> CTCCTCTTC;> GA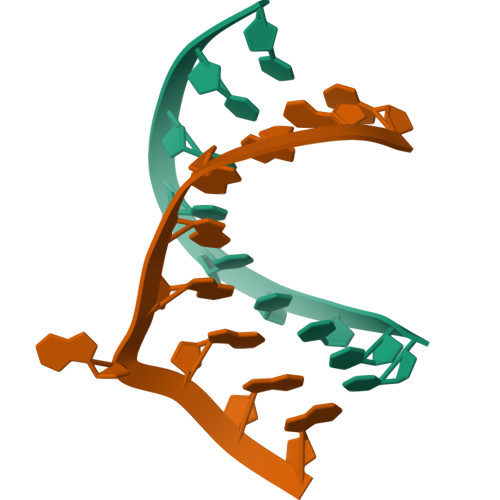AGAGAGAG> HHHHHHHHGEVVSQRYPPAPGLLKYLEQDVCYSLYYYLNWTSLADCKTNFEETGISDVPSTVKVRCQSKNSIRFETEPSEHWQLFILMEHDNFDPIPFTLIEPNNVFGELITTANKEYQIWSTYLDEYGTLQDWMEGPIVLKFDQRNQQPDDIKYNVTQEFKYIILGNDSYTINGKFVWNTTGDRDLCFDIANICQNTNMKHAK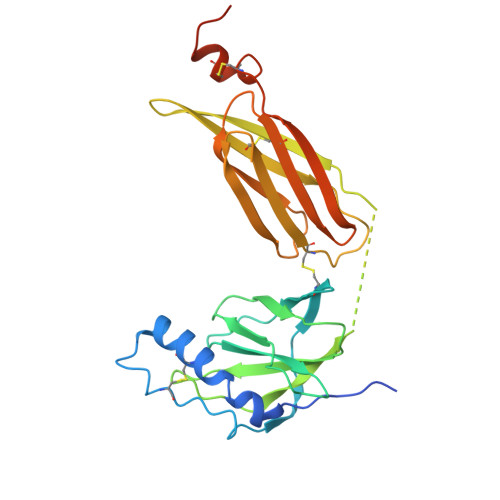IWPTAHPSFDVENLVLNDECEIHVKGIHGTTKHKYKTPSCFELPECFLNNMEPEIPQDVAIAADQDLR Expanding this pattern to hpphhph can produce larger α-helical barrels. Here, we show that pentameric to nonameric barrels are accessed by varying the residue at one of the h sites. In peptides with four L/I–K–E–I–A–x–Z repeats, decreasing the size of Z from threonine to serine to alanine to glycine gives progressively larger oligomers. X-ray crystal structures of the resulting α-helical barrels rationalize this: side chains at Z point directly into the helical interfaces, and smaller residues allow closer helix contacts and larger assemblies.

Whereas, the Gly@g variant with a = Leu, d = Ile had the beginnings of a thermal unfolding curve consistent with the anticipated destabilizing effect of Gly on α-helical structures. The Gly@g peptide with a = Leu, d = Ile crystallized in two forms. Although there are natural nonameric protein assemblies, this is the first stand-alone, water-soluble α-helical CC of this size. The second crystal form revealed a collapsed C2-symmetric 6-helix bundle (Table S4†). We posit that the small size of Gly relaxes this design rule allowing access to other nearby regions of the CC free-energy landscape. The first challenge is incorporating multistate design into αHBs, i.e. considering multiple conformations and/or assemblies that may become accessible in the CC free-energy landscape. However, this becomes difficult with increasing off-target states, e.g. collapsed and anti-parallel structures.

>[6x]XGEIAQGLKEIAKGLKEIAYGLKEIAQGLKGX>MKSKMDPEVTEDGTLELFIRYESKDYINVPTPKVYLNDWTTRERLPIKYNTVQRSKDQLFKSTLTIKDTCYSSSLWAKSKRN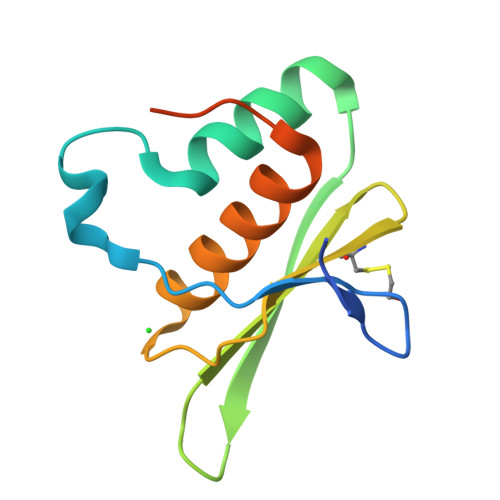AEQSAAMVALEIIGIKTPQSTASNSHHHHHH[2x]> MLQCYNCPNPTADCKTAVNCSSDFDACLITKAGLQVYNKCWKFEHCNFNDVTTRLR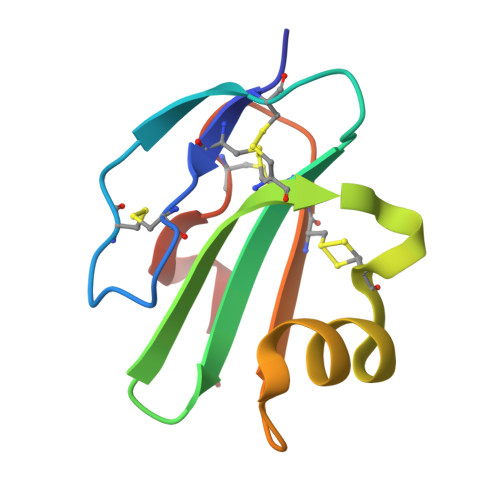ENELTYYCCKKDLCNFNEQLENG> MASINLIKSLKLYKEKIWSFDFSQGILATGSTDRKIKLVSVKYDDFTLIDVLDETAHKKAIRSVAWRPHTSLLAAGSFDSTVSIWAKEESADRTFEMDLLAIIEGHENEVKGVAWSNDGYYLATCSRDKSVWIWETDESGEEYECISVLQEHSQDVKHVIWHPSEALLASSSYDDTVRIWKDYDDDWECVAVLNGHEGTVWSSDFDKTEGVFRLCSGSDDSTVRVWKY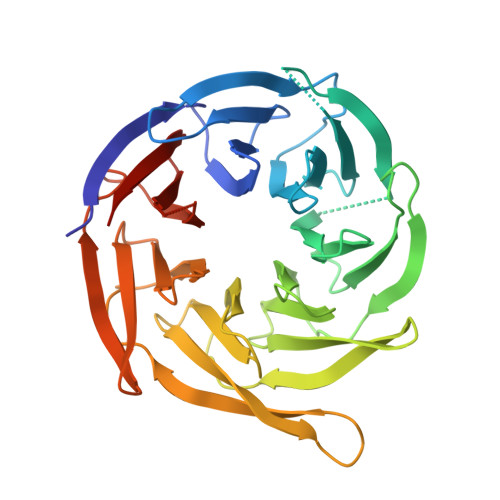MGDDEDDQQEWVCEAILPDVHKRQVYNVAWGFNGLIASVGADGVLAVYEEVDGEWKVFAKRALCHGVYEINVVKWLELNGKTILATGGDDGIVNFWSLEKAA> MDQECIENYAKVNGIYIYYKLCKAPEEKAKLMTMHGGPGMSHDYLLSLRDMTKEGI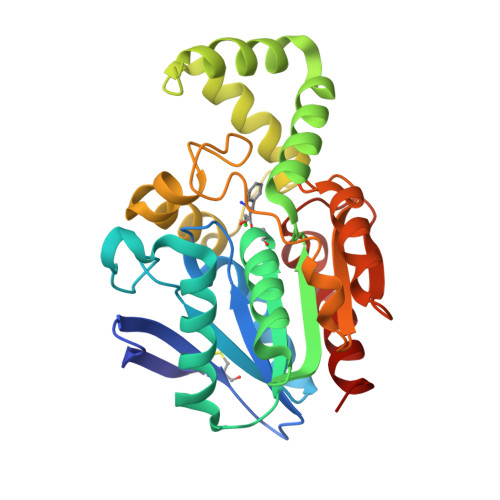TVLFYDQFGCGRSEEPDQSKFTIDYGVEEAEALRSKLFGNEKVFLMGSSYGGALALAYAVKYQDHLKGLIVSGGLSSVPLTVKEMNRLIDELPAKYRDAIKKYGSSGSYENPEYQEAVNYFYHQHLLRSEDWPPEVLKSLEYAERRNVFRIMNGPNEFTITGTIKDWDITDKISAIKIPTLITVGEYDEVTPNVARVIHEKIAGSELHVFRDCSHLTMWEDREGYNKLLSDFILKHL>GPLLKLFDISIL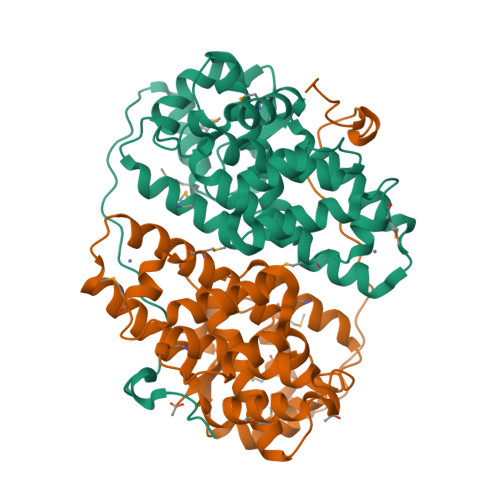PKSGEPKLFLPVPSLPCQEAEKTNDKYVLAMAQRAMHDVPISSKQLTANLLPVKFKPLLSIVRYTPNYYYWVSMRKETIASANLCTVAAFLDESLCWGQQYLKNDFIFSENGKDIILDTSSALLSQLVHKIKMLPFCHCLMQTTPQDHIVKQVCYLIASNNRILDAVRYLQTSVIKSPIVLLLAYAVCLPAAIICTKNETQLYSHCMRILKEYRPGDVMNILHESLTQHLNKCPSSTCAYTTRAIVGTKANTTGLFFLPTQ[2x]>MPFVDLEVPTMTTPTPAATPARPRVLTGDRPTGALHLGHLAGSLQNRVRLQDEAELFVLLADVQALTDHFDRPEQVRENVLAVALDYLAAGLDPQKTTCVVQSAVPELAELTVYFLNLVTVSHLRQNPTVKAEIAQKGYGERVPAGFFVYPVSQAADIAAFGATLVPVGDDQLPMLEQTREIVRRFNALYAPVLAEPQAQLSRVPRLPGLDGQAKMSKSLGNAIALGDSADEVARKVMGMYTDPGHLRASDPGRVEGNPVFTFLDAFDPDPARVQALKDQYRAGGLGDVKVKKHLIDVLNGVLAPIRTRR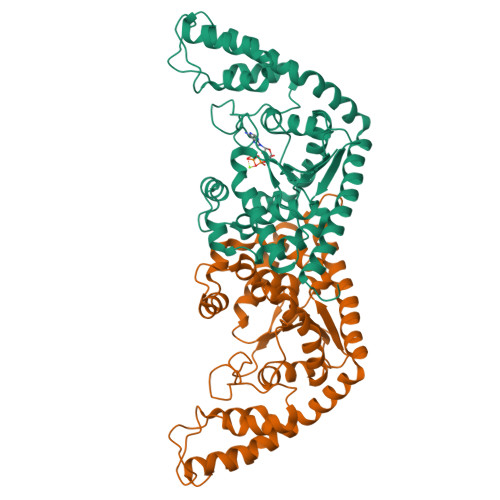AEYERDPDAVLRFVTEGTARGREVAAQTLGQVRRAMRLFGH[3x]>MDLKDSVVSDTFELRPVIGLTRGLSSADIETLTANAIRLHRQLLEKADQLFQVLPDDIKIGTAAGGEQHLEYIEAMIEMHAQMSAVN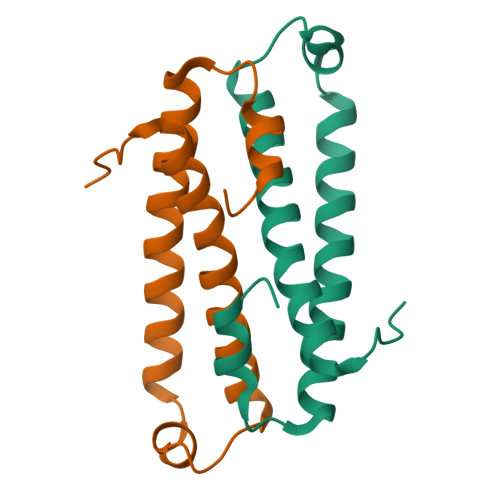TLVGLLGFIPKVSVN[4x]>MVLYFIGLGLYDERDITVKGLEIAKKCDYVFAEFYTSLMAGTTLGRIQKLIGKKIRVLSREDVELNFENIVLPLAKENDVAFLTPGDPLVATTHAELRIRAKRAGVESYVIHAPSIYSAVGITGLHIYKFGKSATVAYPEGNWFPTSYYDVIKENAERGLHTLLFLDIKAEKRMYMTANEAMELLLKVEDMKKGGVFTDDTLVVVLARAGSLNPTIRAGYVKDLIREDFGDPPHILIVPGKLHIVEAEYLVEIAGAPREIL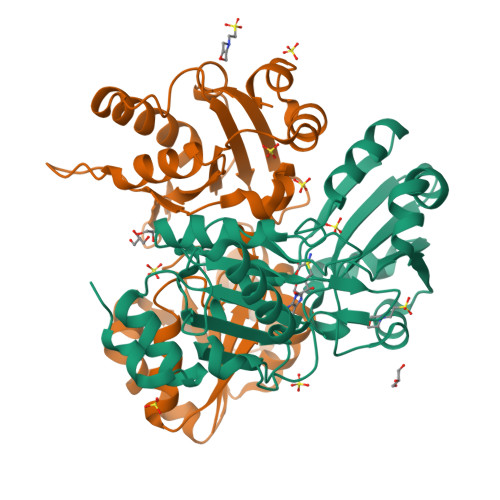RVNV[2x]> MAHHHHHHYVEEKKEIDSLMEDVLALVNDSSGGKF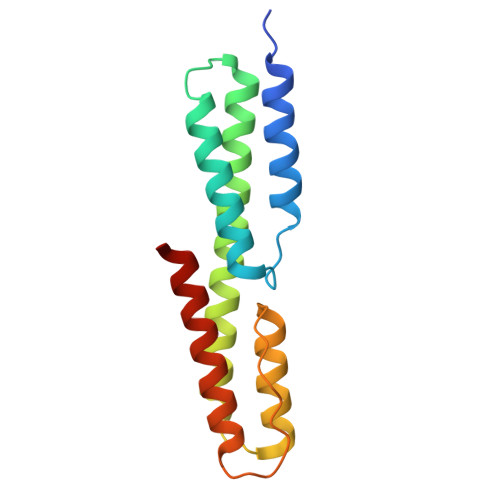KDYKDKINELKENLKDIGNAELKEKLLNLQNSFQDKLAAKLAALKAAKNTIENITDKDQDISKRKIWSEAKLVGVTVPLLGSNTSGNGDKMSKNAVEQIDKVIKFLEEGTN> GSHMANLDRTDDLVYLNVMELVRAVLELKNELSQLPPEGYVVVVKNVGLTLRKLIGSVDDLLPSLPSSSRTEIEGTQKLLNKDLAELINKMRLAQ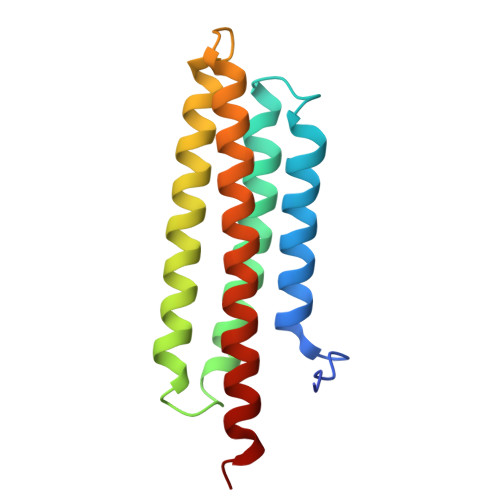QNAVTSLSEEAKRQMLTASHTLAVDAKNLLDAVDQAKVLANLAH>GSHMVERISLEKAALEFSEANAPHPRIYELPVEEGRSLLNEVQDSPVVKEDVDIEDIAVDTGEWGEINVRFIRPLHQEKKLPVIFYIHGAGWVFGNAHTHDKLIRELAVRTNSVVVFSEYSLSPEAKYPTAIEQNYAVLQQLKDFANDKKFDVNHLTVAGDSVGGNMATVMTLLTKQRGGQKIGQQVLYYPVTDANFDTDSYNEFAENYFLTKEGMIWFWDQYTTSQEERHQITASPLRATKEDLADLPAALIITGEADVLRDEGEAYARKLREADVEVTQVRFQAIIHDFVMVNSMNETHATRAAMSLSTQWINEKNRK[3x]

In this study, we performed an in-depth biochemical and structural characterization of a novel microbial acetylesterase, LgEstI, from the bacterial fish pathogen Lactococcus garvieae. LgEstI belongs to the HSL family of α/β-hydrolases and presents a clear substrate preference for a short acyl chain and an acetate moiety that are suitable for the narrow entrance to the active site. Monomeric LgEstI exhibits a canonical α/β hydrolase fold with conserved key active site residues. The active site of LgEstI has the typical catalytic triad of esterases, identified as Ser159, Asp256, and His286, and is located at the bottom of the substrate access channel.

The three-dimensional structure of LgEstI was determined using X-ray crystallography at 2.0 Å resolution. An LgEstI crystal contained three monomers per asymmetric unit. Superposition analysis revealed that each monomer was almost identical, with a root-mean-square deviation (RMSD) of ~ 0.3 Å (Cα), including most of the water molecules surrounding the monomers. The monomer can be divided into two domains: a CAP domain and an α/β hydrolase domain. The CAP domain is made up of three triangular helices, α1, α2, and α8, whereas the α/β hydrolase domain consists of a 90-degree twisted β sheet in the center, five neighboring α-helices (α3, α4, α6, α10, and α11), and turns connecting helices and strands. Careful investigation of the active site of wild-type LgEstI indicated that two of the three monomers had a triangular blob at the tip of the hydroxyl group of Ser159. The crystallization condition included 0.1 M calcium acetate hydrate; therefore, we incorporated acetate into the blob as it had a 0.5 reasonable density fit value. The acetate moiety was positioned at the bottom of the active site and surrounded by Val160, Met213, His286, and Asp287 within hydrogen bonding distances, and an oxyanion hole consisting of Ala87 and Gly88. The oxygen atom interacts with the NE2 of His286, and the methyl group of acetate is directed toward Val160 for hydrophobic interactions. Unlike other esterases, LgEstI contains bulky residues such as Trp89, Phe194, and Trp217, which block the acyl chain channel.>MQFEHLVQVNDRTLVDLPVLDRLQLWEG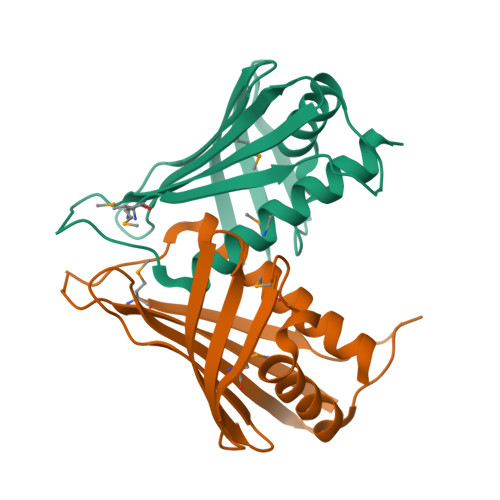LVCRAREPQYFVVGLERFEILVDDGDRLHRRLYLPGLVVEDEVVLKAPDSAHYSIKPSAEVAGGSLDMTIEEPEPGSLFVRFAYCTRYLQPLGDELPYDAFVKQAYIAMDVETIATIRDRFGASAASGS[2x]1-[2-(3-BIPHENYL)-4-METHYLVALERYL)]AMINO-3-(2-PYRIDYLSULFONYL)AMINO-2-PROPANONE 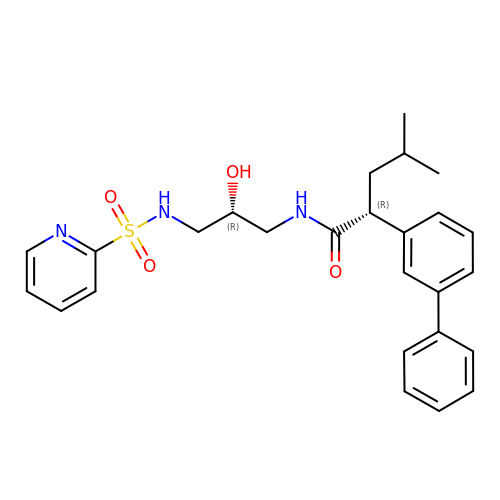| C26 H31 N3 O4 S | YCDHZDINQZLSRR-DNQXCXABSA-N> GHMSQSNRELVVDFLSYKLSQKGYSWSQFSDVEENRTEAPEETEAERETPSAINGNPSWHLADSPAVNGATGHSSSLDAREVIPESAVKQALREAGDEFELRYRRAFSDLTSQLHITPGTAYQSFEQVVNELFRDGVNWGRIVAFFSFGGALCVESVDKEMQVLVSR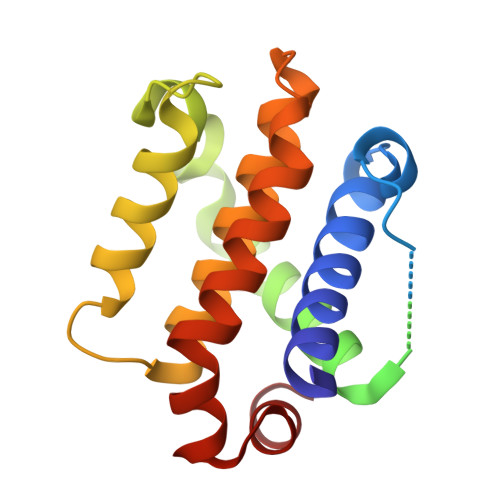IASWMATYLNDHLEPWIQENGGWDTFVDLYG> GSHMSSLPVPYKLPVSLSVGSCVIIKGTPIH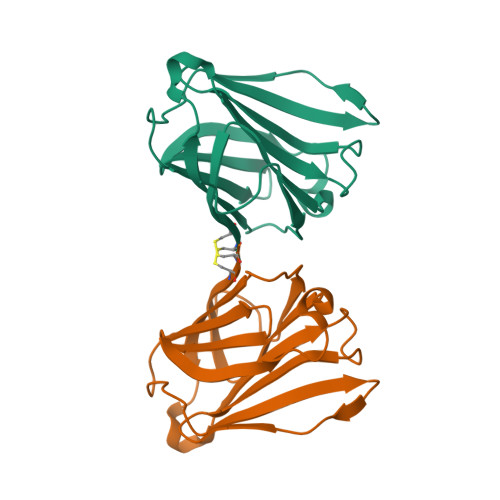SFINDPQLQVDFYTDMDEDSDIAFRFRVHFGNHVVMNRREFGIWMLEETTDYVPFEDGKQFELCIYVHYNEYEIKVNGIRIYGFVHRIPPSFVKMVQVSRDISLTSVCVCN> MAMHPRKDWYELTRATNWTPSYVTEEQLFPERMSGHMGIPLEKWESYDEPYKTSYPEYVSIQREKDAGAYSVKAALERAKIYENSDPGWISTLKSHYGAIAVGEYAAVTGEGRMARFSKAPGNRNMATFGMMDELRHGQLQLFFPHEYCKKDRQFDWAWRAYHSNEWAAIAAKHF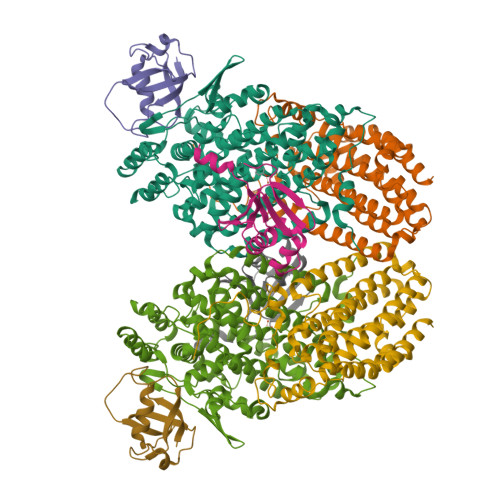FDDIITGRDAISVAIMLTFSFETGFTNMQFLGLAADAAEAGDYTFANLISSIQTDESRHAQQGGPALQLLIENGKREEAQKKVDMAIWRAWRLFAVLTGPVMDYYTPLEDRSQSFKEFMYEWIIGQFERSLIDLGLDKPWYWDLFLKDIDELHHSYHMGVWYWRTTAWWNPAAGVTPEERDWLEEKYPGWNKRWGRCWDVITENVLNDRMDLVSPETLPSVCNMSQIPLVGVPGDDWNIEVFSLEHNGRLYHFGSEVDRWVFQQDPVQYQNHMNIVDRFLAGQIQPMTLEGALKYMGFQSIEEMGKDAHDFAWADKCK;> MSFESKKPMRTWSHLAEMRKKPSEYDIVSRKLHYSTNNPDSPWELSPDSPMNLWYKQYRNASPLKHDNWDAFTDPDQLVYRTYNLMQDGQESYVQSLFDQFNEREHDQMVREGWEHTMARCYSPLRYLFHCLQMSSAYVQQMAPASTISNCCILQTADSLRWLTHTAYRTHELSLTYPDAGLGEHERELWEKEPGWQGLRELMEKQLTAFDWGEAFVSLNLVVKPMIVESIFKPLQQQAWENNDTLLPLLIDSQLKDAERHSRWSKALVKHALENPDNHAVIEGWIEKWRPLADRAAEAYLSMLSSDI;> MSAFPVHAAFEKDFLVQLVVVDLNDSMDQVAEKVAYHCVNRRVAPREGVMRVRKHRSTELFPRDMTIAESGLNPTEVIDVVFEE;> MSTLADQALHNNNVGPIIRAGDLVEPVIETAEIDNPGKEITVEDRRAYVRIAAEGELILTRKTLEEQLGRPFNMQELEINLASFAGQIQADEDQIRFYFDKTM>RKPKTGILMLNMGGPETLGDVHDFLLRLFLDRDLMTLPIQNKLAPFIAKRRTPKIQEQYRRIGGGSPIKIWTSKQGEGMVKLLDELSPNTAPHKYYIGFRYVHPLTEEAIEEMERDGLERAIAFTQYPQYSCSTTGSSLNAIYRYYNQVGRKPTMKWSTIDRWPTHHLLIQCFADHILKELDHFPLEKRSEVVILFSAHSLPMSVVNRGDPYPQEVSATVQKVMERLEYCNPYRLVWQSKVGPMPWLGPQTDESIKGLCERGRKNILLVPIAFTSDHIKTLYELDIEYSQVLAKECGVENIRRAESLNGNPLFSKALADLVHSHIQSNELCSKQLTLSC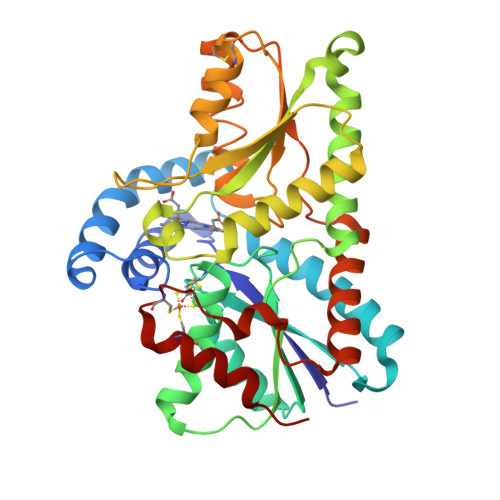PLCVNPVCRETKSFFTSQQL[4x]>MGHHHHHHSHMPVTEKDLAEDAPWKKIQQNTFTRWCNEHLKCVNKRIGNLQTDLSDGLRLIALLEVLSQKRMYRKYHQRPTFRQMQLENVSVALEFLDRESIKLVSIDSKAIVDGNLKLILGLVWTLILHYSISMP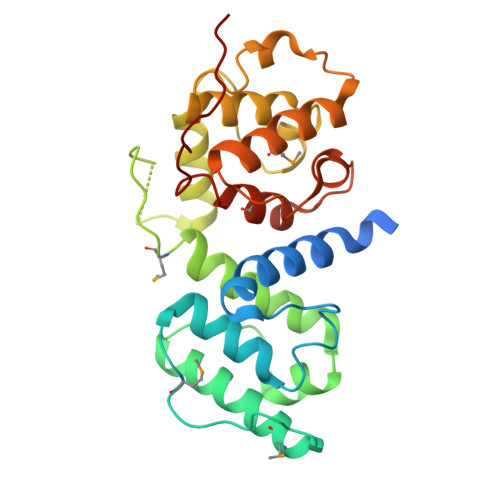VWEDEGDDDAKKQTPKQRLLGWIQNKIPYLPITNFNQNWQDGKALGALVDSCAPGLCPDWESWDPQKPVDNAREAMQQADDWLGVPQVITPEEIIHPDVDEHSVMTYLSQFPKAKLKPGAPLKPKL[4x]>MKTMRKQIYKKAYWLLLPFLPLALANTFLVKEDSKNVTAYTPFATPITDSKSDLVSLAQLDSSYQIADQTIHNTNLFVLFKSRDVKVKYESSGSNNISFDSTSQGEKPSYVVEFTNSTNIGIKWTMVKKYQLDVPNVSSDMNQVLKNLILEQPLTKYTLNSSLAKEKGKTQREVHLGSGQANQWTSQRNQHDLNNNPSPNASTGFKLTTGNAYRKLSESWPIYEPIDGTKQGKGKDSSGWSSTEENEAKNDAPSVSGGGSSSGTFNKYLNTKQALESIGILFDDQTPRNVITQLYYASTSKLAVTNNHIVVMGNSFLPSMWYWVVERSAQENASNKPTWFANTNLDWGEDKQKQFVENQLGYKETTSTNSHNFHSKSFTQPAYLISGIDSVNDQIIFSGFKAGSVGYDSSSSSSSSSSSSTKDQALAWSTTTSLDSKTGYKDLVTNDTGLNGPINGSFSIQDTFSFVVPYSGNHTNNGTTGPIKTAYPVKKDQKSTVKINSLINATPLNSYGDEGIGVFDALGLNYNFKSNQERLPSRTDQIFVYGIVSPNELRSAKSSADSTGSDTKVNWSNTQSRYLPVPYNYSEGIIDADGFKRPENRGASVTTFSGLKSIAPDGFANSIANFSVGLKAGIDPNPVMSGKKANYGAVVLTRGGVVRLNFNPGNDSLLSTTDNNIAPISFSFTPFTAAESAVDLTTFKEVTYNQESGLWSYIFDSSLKPSHDGKQTPVTDNMGFSVITVSRTGIELNQDQATTTLDVAPSALAVQSGIQSTTQTLTGVLPLSEEFSAVIAKDSDQNKIDIYKNNNGLFEIDTQLSNSVATNNGGLAPSYTENRVDAWGKVEFADNSVLQARNLVDKTVDEIINTPEILNSFFRFTPAFEDQKATLVATKQSDTSLSVSPRIQFLDGNFYDLNSTIAGVPLNIGFPSRVFAGFAALPAWVIPVSVGSSVGILFILLVLGLGIGIPMYRVRKLQDASFVNVFKKVDTLTTAVGSVYKKIITQTGVVKKAPSALKAANPSVKKPAAFLKPPVQPPSKPEGEQKAVEVKSEETKS[2x];>MHQPKKRLAKKSWAFLTAALTLGVITGVGGYFLFNQNKQRSSVSNFAYQPKQLSVKHQQAVDETLTPWTWNNNNFSSLKITGENPGSFGLVRSQNDNLNISSVTKNSSDDNLKYLNAVEKYLDGQQNFAIRRYDNNGRALYDINLAKMENPSTVQRGLNGEPIFDPFKGFGLTGNAPTDWNEIKGKVPVEVVQSPHSPNLYFVLLVPKVALEYHNLNNQVVKESLEVKATQSSFNPTQRLQKDSPVKDSSKQGEKLSETTASSMSSGMATSTRAKALKVEVERGSQSDSLLKNDFAKKPLKHKNSSGEVKLEAEKEFTEAWKPLLTTDQIAREKGMGATVVSFYDAPYSENHTAFGLVDHIDPKKMVENYPPSWKTPKWNHHGIWDYNARNLLLQTTGFFNPRRHPEWFDEGQAKADNTSPGFKVGDTDHKKDGFKKNSSSPIALPFEAYFANIGNMVAIGNSVFIFGGNGHATKMFTTNPLSIGVFRIKYTDNFSKSSVTGWPYAVLFGGLINPQTNGLKDLPLGTNRWFEYVPRMAVSGVKWVGNQLVLAGTLTMGDTATVPRLKYDQLEKHLNLVAQGQGLLREDLQIFTPYGWANRPDIPVGAWLQDEMGSKFGPHYFLNNPDIQDNVNNDTVEALISSYKNTDKLKHVYPYRYSGLYAWQLFNWSNKLTNTPLSANFVNENSYAPNSLFAAILNEDLLTGLSDKIFYGKENEFAENEADRFNQLLSLNPNPNTNWARYLNVVQRFTTGPNLDSSTFDQFLDFLPWIGNGKPFSNSPSPSTSASSSTPLPTFSNINVGVKSMITQHLNKENTRWVFIPNFSPDIWTGAGYRVQSANQKNGIPFEQVKPSNNSTPFDPNSDDNKVTPSGGSSKPTTYPALPNSISPTSDWINALTFTNKNNPQRNQLLLRSLLGTIPVLINKSGDSNDQFNKDSEQKWDKTETNEGNLPGFGEVNGLYNAALLHTYGFFGTNTNSTDPKIGFKADSSSSSSSTLVGS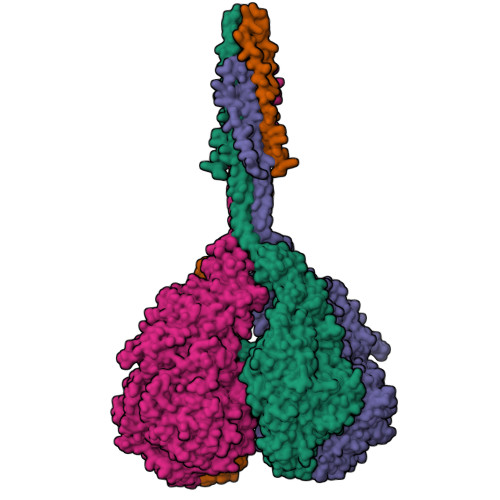GLNWTSQDVGNLVVINDTSFGFQLGGWFITFTDFIRPRTGYLGITLSSLQDQTIIWADQPWTSFKGSYLDSDGTPKSLWDPTALKSLPNSSTTYDTNPTLSPSFQLYQPNKVKAYQTTNTYNKLIEPVDATSAATNMTSLLKLLTTKNIKAKLGKGTASSQGNNNGGGVSQTINTITTTGNISEGLKEETSIQAETLKKFFDSKQNNKSEIGIGDSTFTKMDGKLTGVVSTPLVNLINGQGATSDSDTEKISFKPGNQIDFNRLFTLPVTELFDPNTMFVYDQYVPLLVNLPSGFDQASIRLKVISYSVENQTLGVRLEFKDPQTQQFIPVLNASSTGPQTVFQPFNQWADYVLPLIVTVPIVVIILSVTLGLTIGIPMHRNKKALQAGFDLSNKKVDVLTKAVGSVFKEIINRTGISNAPKKLKQATPTKPTPKTPPKPPVKQ[2x]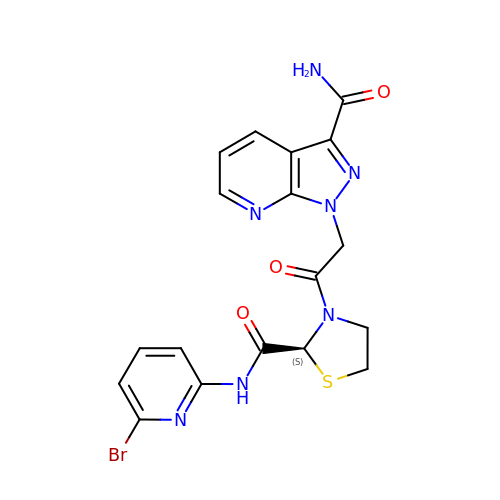1-(2-{(2S)-2-[(6-bromopyridin-2-yl)carbamoyl]-1,3-thiazolidin-3-yl}-2-oxoethyl)-1H-pyrazolo[3,4-b]pyridine-3-carboxamide | C18 H16 Br N7 O3 S | AOOWOKALXAVACG-SFHVURJKSA-N> ANNLGSKLLVGYWHNF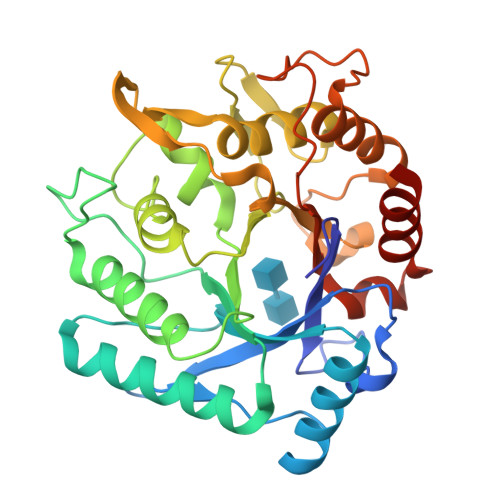DNGTGIIKLKDVSPKWDVINVSFGETGGDRSTVEFSPVYGTDADFKSDISYLKSKGKKVVLSIGGQNGVVLLPDNAAKDRFINSIQSLIDKYGFDGIDIDLQSGIYLNGNDTNFKNPTTPQIVNLISAIRTISDHYGPDFLLSMAPETAYVQGGYSAYGSIWGAYLPIIYGVKDKLTYIHVQHFNAGSGIGMDGNNYNQGTADYEVAMADMLLHGFPVGGNANNIFPALRSDQVMIGLPAAPAAAPSGGYISPTEMKKALNYIIKGVPFGGKYKLSNQSGYPAFRGLMSWSINWDAKNNFEFSNNYRTYFDGLSLQK Overexpression of NAMPT has been observed in different cancer types and has been implicated to confer resistance to classic chemotherapeutics, whereas inhibition sensitizes cancer cells to oxidative stress and DNA-damaging agents. Thus, inhibition of NAD+ biosynthesis facilitated by NAMPT shows potential as an anticancer therapy. KPT-9274 represents a new class of NAMPT inhibitors and shows promising pharmacokinetics (Karyopharm Therapeutics). Using the CRISPRres approach, we revealed NAMPT as the key cellular target of the clinical inhibitor KPT-9274 by showing that mutations in NAMPT confer resistance to KPT-9274.

Crystallographic analysis of the binding mode revealed that two KPT-9274 molecules are bound to the NAMPT dimer. The binding mode is largely similar to that of FK866. In more detail, the amino-pyridinyl of KPT-9274 is coordinated via pi-stacking interactions between tyrosine 18 and phenylalanine 193. Furthermore, the amide linker is well coordinated via hydrogen-bonding interactions and the free electron pairs of the amide oxygen are stabilized by a hydrogen bond originating from serine 275. The nitrogen forms a hydrogen bond with a water molecule that further interacts with the carboxyl group of aspartate 219 and the hydroxyl group of serine 241. At the solvent exposed regions of the binding site, the chemical composition of KPT-9274 and the interactions with the NAMPT protein are different from FK866. KPT-9274 is branched and binds to two different solvent exposed patches whereas FK866 only occupies a single hydrophobic site. The first hydrophobic patch outlined by the hydrophobic sidechains of isoleucine 309, isoleucine 351, and alanine 379 is occupied by the aromatic fluorophenyl group of KPT-9274. The second solvent exposed binding site, which is only covered by KPT-9274, consists of tyrosine 188 and tyrosine 240 that interact with the difluoro-1-piperidinyl carbonyl phenyl group via Van der Waals interactions and a hydrogen bond between the carbonyl group and the amino group of lysine 216. Deletion of G383 causes a conformational change of the G383–385 stretch, which destablizes the conformation of F193 and thereby prevents pi-stacking with the ligand.

>[2x]MNPAAEAEFNILLATDSYKVTHYKQYPPNTSKVYSYFECREKKTENSKLRKVKYEETVFYGLQYILNKYLKGKVVTKEKIQEAKDVYKEHFQDDVFNEKGWNYILEKYDGHLPIEIKAVPEGFVIPRGNVLFTVENTDPECYWLTNWIETILVQSWYPITVATNSREQKKILAKYLLETSGNLDGLEYKLHDFGYRGVSSQETAGIGASAHLVNFKGTDTVAGLALIKKYYGTKDPVPGYSVPAAEHSTITAWGKDHEKDAFEHIVTQFSSVPVSVVSDSYDIYNACEKIWGEDLRHLIVSRSTQAPLIIRPDSGNPLDTVLKVLEILGKKFPVTENSKGYKLLPPYLRVIQGDGVDINTLQEIVEGMKQKMWSIENIAFGSGGGLLQKLTRDLLNCSFKCSYVVTNGLGINVFKDPVADPNKRSKKGRLSLHRTPAGNFVTLEEGKGDLEEYGQDLLHTVFKNGKVTKSYSFDEIRKNAQLNIELEAAHHENLYFQ> MKRKTAEVKGEKERNSKQISLEEDKIKGMFNPKIWDKTFQDGLKKEIEDSQPYNWGTIHELVNDDLLRAVRKEIETEIHFTKKETDIYRVNQSGDLANLSGLDWDDLSRLPNLFKLRQILYSKQYRDFFGYVTKAGKLSGSKTDMSINTYTKGCHLLTHDDVIGSRRISFILYLPDPDRKWKSHYGGGLRLFPSILPNVPHSDPSAKLVPQFNQIAFFKVLPGFSFHDVEEVKVDKHRLSIQGWYHIPQVGEEGYIPGEEEAWVRNNTSTLAQIESNVLEDFEFPKDERNILSFHEVKHFEKMLKGDAGAKTDNTPKESMTSVISDSVKLSEAEFTYLSQYISPEHLSSKGIEKLQKQFVENSSLQIESFLNDDKSELLKKVIKQKELEQECPYHSKDVKAPWKTAIPPHKARYLYIDGKEYRNFQTEADILEALNNNDLPNFQFTKDAIKIISDASGNSREN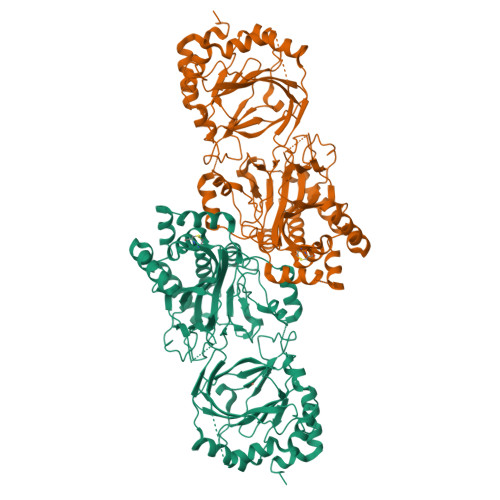NFDAELALIDLAVFHKSTIFKKYLALLTSLCPVSEQILIRRFRPGMDFTLATKCRFNELLKSNPDIIDAVLEGTLCLTPSAGWESGELGGYELYMMDDDEDNKQYLKEDVEDASVYRADDSGDSVLINDPPAWNTFNLVLRDESVLEFVKYVSWSAKSSRWDVKMKWDVKSCDEDGQEDEA>MASVQLQNVTKAWGEVVVSKDINLDIHEGEFVVFVGPSGCGKSTLLRMIAGLETITSGDLFIGEKRMNDTPPAERGVGMVFQSYALYPHLS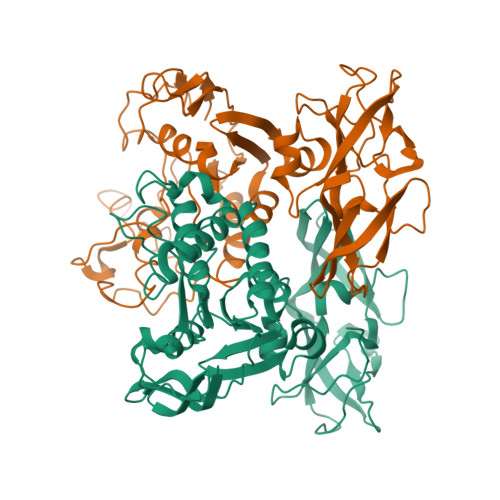VAENMSFGLKLAGAKKEVINQRVNQVAEVLQLAHLLDRKPKALSGGQRQRVAIGRTLVAEPSVFLLDEPLSNLDAALRVQMRIEISRLHKRLGRTMIYVTHDQVEAMTLADKIVVLDAGRVAQVGKPLELYHYPADRFVAGFIGSPKMNFLPVKVTATAIDQVQVELPMPNRQQVWLPVESRDVQVGANMSLGIRPEHLLPSDIADVILEGEVQVVEQLGNETQIHIQIPSIRQNLVYRQNDVVLVEEGATFAIGLPPERCHLFREDGTACRRLHKEPGVESASHHHHHH[4x]> MQQASTPTIGMIVPPAAGLVPADGARLYPDLPFIASGLGLGSVTPEGYDAVIESVVDHARRLQKQGAAVVSLMGTSLSFYRGAAFNAALTVAMREATGLPCTTMSTAVLNGLRALGVRRVALATAYIDDVNERLAAFLAEESLVPTGCRSLGITGVEAMAR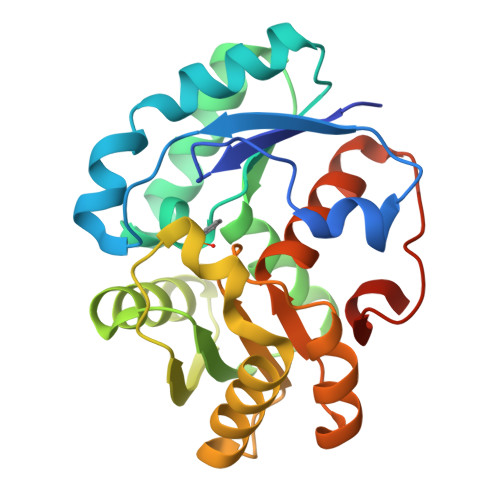VDTATLVDLCVRAFEAAPDSDGILLSCGGLLTLDAIPEVERRLGVPVVSSSPAGFWDAVRLAGGGAKARPGYGRLFDESLEHHHHHH>[2x]GMKLQTTIQHEPKDGSGFDRGLREFFEYRDTGVNEATGGMFGAHVIRAIPGKEAKPTWHTHTVGFQLFYVLRGWVEFEYEDIGAVMLEAGGS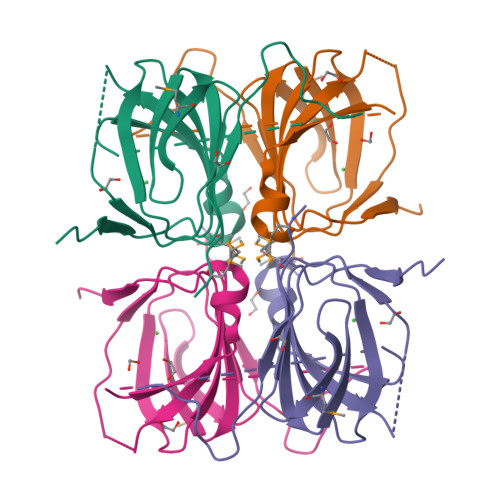AFQPPGVRHRELRHSDDLEVLEIVSPAGFATSVVDLEEARKP(3S,5E)-3-propyl-3,4-dihydrothieno[2,3-f][1,4]oxazepin-5(2H)-imine 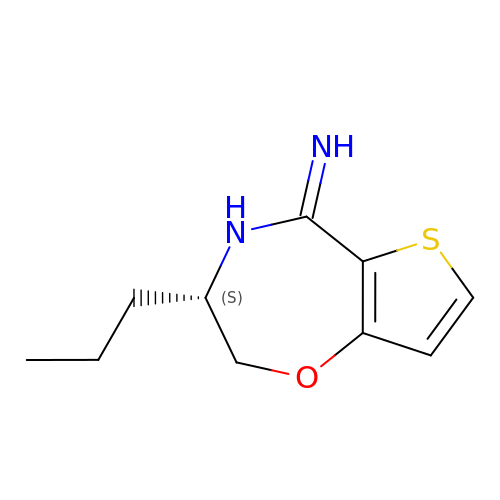| C10 H14 N2 O S | JIIBOYBTIWHZFJ-ZETCQYMHSA-N>[2x]MDYMYGPGRHHLFVPGPVNIPEPVIRAMNRNNEDYRSPAIPALTKTLLEDVKKIFKTTSGTPFLFPTTGTGAWESALTNTLSPGDRIVSFLIGQFSLLWIDQQKRLNFNVDVVESDWGQGANLQVLASKLSQDENHTIKAICIVHNETATGVTNDISAVRTLLDHYKHPALLLVDGVSSICALDFRMDEWGVDVALTGSQKALSLPTGLGIVCASPKALEATKTSKSLKVFFDWNDYLKFYKLGTYWPYTPSIQLLYGLRAALDLIFEEGLENIIARHARLGKATRLAVEAWGLKNCTQKEEWISNTVTAVMVPPHIDGSEIVRRAWQRYNLSLGLGLNKVAGKVFRIGHLGNVNELQLLGCLAGVEMILKDVGYPVVMGSGVAAASTYLQHHIPLIPSRI

The alanine:glyoxylate aminotransferase 1 (AGT1) gene (At2G13360) of Arabidopsis encodes a multifunctional class IV aminotransferase protein that catalyzes transamination reactions using l-serine, l-alanine, and l-asparagine as amino donors and glyoxylate, pyruvate, and hydroxypyruvate as amino acceptors. The tertiary structure of Arabidopsis AGT1 is characteristic of the subgroup IV class of PLP-containing enzymes. A prior study of Arabidopsis AGT1 demonstrated that the active enzyme exists as a dimer. The reaction mechanism of human AGT1 has been described in detail, and because the catalytic residues are conserved in Arabidopsis AGT1, this protein likely has the same mechanism.

Here we describe the structure of AGT1 from Arabidopsis thaliana, solved using X-ray crystallography at a resolution of 2.1 Å, and highlight the molecular determinants of its substrate specificity. The results described herein are for the AGT1 crystals grown in the presence of l-serine and are valid for both structures unless explicitly mentioned. Molecules from each crystal form were almost identical; root mean square distance between α-carbon atoms was 0.10 Å for 798 α-carbons. In the AGT1 structure crystallized in the presence of l-serine, a pyridoxamine phosphate (PMP) molecule and no internal aldimine bond were expected, but the geometry and close distance of the PMP amino group (N4A) to the Lys201 NZ suggested that the cofactor should best be modeled as PLP. l-Serine molecule (magenta) was modeled in AGT1 guided by the difference density in (A). The l-serine hydroxyl group is within hydrogen-bonding distance of Tyr35′, Arg36′, and a water molecule. The Tyr260′ aromatic ring may sterically clash with the hydroxyl of l-serine. Indeed, these two residues are highly conserved among a wide range of known and putative plant serine:glyoxylate amino transferases. Data for both crystals were collected at room temperature.> GSHMASRENEMDENLEQVSGIIGNLRHMALDMGNEIDTQNRQI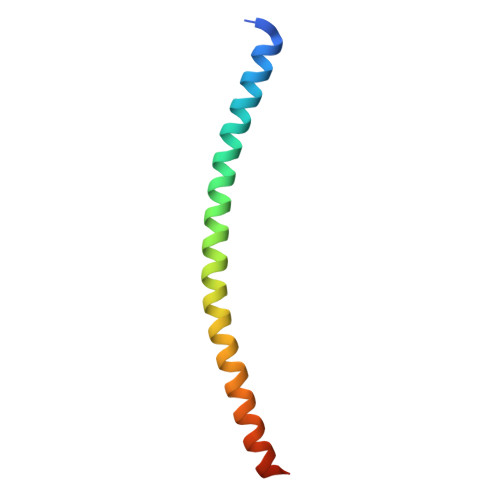DRIMEKADSNKTRIDEANQRATKMLG>[2x]MHHHHHHGSPSRSAEIMKHGYPGFTNVRTYEDFVLSYDYKTRTAHWVCEHLTPERLKHAEGVDRKLCEAKPDITFPQKFLS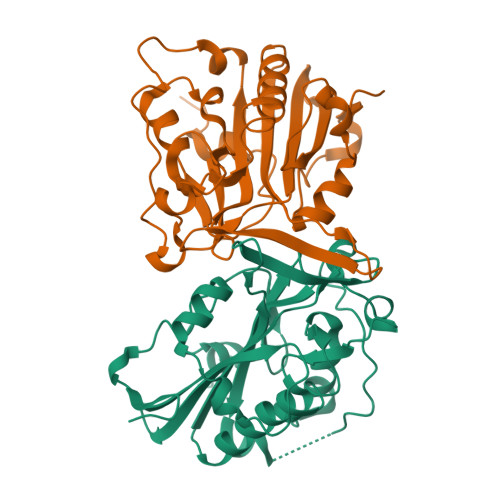QNTDYKCSGFDRGALAAAGNHRKSQLAVDQTFYLSNMSPQVGRGFNRDKWNDLEMHCRRVAKKMINSYIITGPLYLPKLEGDGKKYIKYQVIGDNNVAVPTHFFKVALFEVTPGKFELESYILPNAVIEDTVEISKFHVPLDAVERSAGLEIFARLDPKSIVKENGAKKGG>[6x]MGLPRGSFFWLLLLLTAACSGLLFALYFSAVQRYPGPAAGARDTTSFEAFFQSKASNSWTGKGQACRHL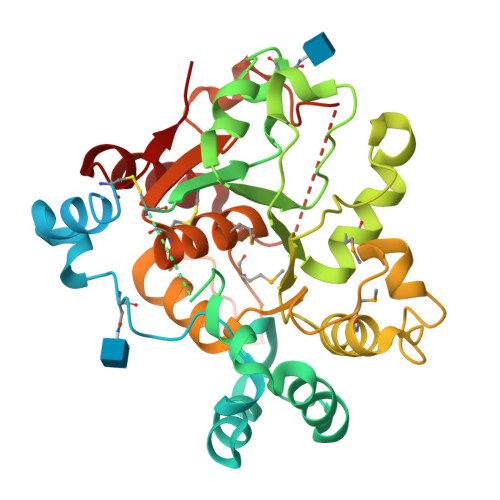LHLAIQRHPHFRGLFNLSIPVLLWGDLFTPALWDRLSQHKAPYGWRGLSHQVIASTLSLLNGSESAKLFAPPRDTPPKCIRCAVVGNGGILNGSRQGPNIDAHDYVFRLNGAVIKGFERDVGTKTSFYGFTVNTMKNSLVSYWNLGFTSVPQGQDLQYIFIPSDIRDYVMLRSAILGVPVPEGLDKGDRPHAYFGPEASASKFKLLHPDFISYLTERFLKSKLINTHFGDLYMPSTGALMLLTALHTCDQVSAYGFITSNYWKFSDHYFERKMKPLIFYANHDLSLEAALWRDLHKAGILQLYQR> EQTSIAHLTSDDVNLPGSDFFRFYRSADKQEKEKARIYLLGVLDATEGKSWCQYSQLQTVTLQEFVFEFFNKLPAARLHERAAPLIEEALAT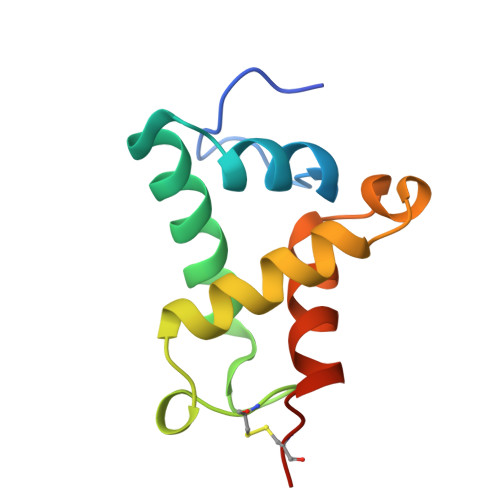RFPCKGGKA> ASITEIKADKTTAVANGQDAITYTVKVMKGDKPVSNQEVTFTTTLGKLSNSTEKTDTNG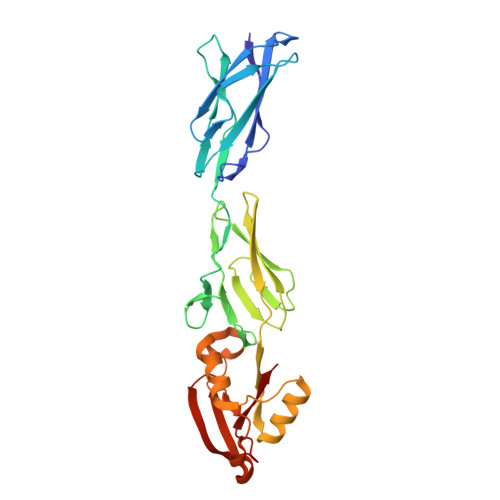YAKVTLTSTTPGKSLVSARVSDVAVDVKAPEVEFFTTLTIDDGNIEIVGTGVKGKLPTVWLQYGQVNLKASGGNGKYTWRSANPAIASVDASSGQVTLKEKGTTTISVISSDNQTATYTIATPNSLIVPNMSKRVTYNDAVNTCKNFGGKLPSSQNELENVFKAWGAANKYEYYKSSQTIISWVQQTAQDAKSGVASTYDLVKQNPLNNIKASESNAYATCVK Periplasmic solute-binding proteins (SBPs) specific for chitooligosaccharides, (GlcNAc)n (n = 2, 3, 4, 5 and 6), are involved in the uptake of chitinous nutrients and the negative control of chitin signal transduction in Vibrios. Here we propose three-domain mechanism of the (GlcNAc)n translocation based on experiments using a recombinant VcCBP, SBP specific for (GlcNAc)n from Vibrio cholerae. X-ray crystal structures of unliganded or (GlcNAc)3-liganded VcCBP solved at 1.2–1.6 Å revealed three distinct domains, the Upper1, Upper2 and Lower domains for this protein. Based on the crystal structures and molecular dynamics simulation, we here propose that the three domains, Upper1, Upper2, and Lower domains, which correspond to domains I, II, and III, respectively, are required to explain the translocation process of (GlcNAc)2 by CBP.

We solved the structure of unliganded protein (open form) at 1.6 Å, a higher resolution than the VcCBP structures formerly deposited (2.2–2.3 Å resolution). The unliganded form exhibited the largest motion (RMSD, 0.8 nm) of the entire protein molecule, while the motions of the individual domains remained at lower levels (RMSD, 0.1–0.3 nm). This clearly indicated a domain motion, in which the individual domains did not change their own conformations but changed their relative arrangement. In unliganded VcCBP, essential subspaces were widely extended as compared with the liganded VcBP (eigenvector1/eigenvector, -7 ~ 15 nm/-22 ~ 9 nm) revealing a large conformational change from the open state to the closed state. In unliganded VcCBP, strong self-positive correlations (red) were found in the region of residue No. 1-239, which corresponds to Upper1 + Upper2 domains, and also in residue No. 350-440, which includes amino acid residues interacting with the ligand from Lower domain. However, strong inter-negative correlations (blue) were found between 1 and 239 (Upper1 + Upper2) and 350–440 (the interacting region of Lower domain). Furthermore, inter-correlations between 140 and 239 (inner Upper1) and 1–35 (N-terminal Upper1) were rather positive (red). It was clear that Upper1 and Upper2 domains move unitedly in the unliganded state, but that these two domains move independently in the (GlcNAc)3-liganded state.

>[2x]MHHHHHHRSELTIVPDFYPTMVRNFNPYLATNLRTTTDFIYEPLVVFNEMKGNTPVFRLAESYKMADDLMSVTFDIRKGVKWSDGEAFTADDVVYSFGLLKAKPELDQRGINKWVTSVEKVDEYKVRFRLSEANSNVPYEISLIPIVAEHVWKDVKDPTTFTNENPVGTGPFTVIDTFTPQLYIQCRNPNYWDAANLEVDCLRVPQIANNDQLLGKIVNSELDWTSSFVPDIDRTYAAANPNHHYWYPAAGTQAFMVNFKNPDPAKKEALDNVDFRRAFSMALDRQTIIDIAFYGSGTVNDFASGLGYAFEAWSDEATHKKYKGFNTYDVEGSKKLLAKAGFKDVNGDGFVETPSGKSFELLIQSPNGWTDFNNTVQLAVEQLQEVGIKAKARTPEFAVYNQAMLEGTYDVAYTNYFHGADPFTYWNSGYNSALQSGDGMPRFAMHYFTDKKLDGLLDSFYKTADKNEQLAIAHGIQKIIAENQVTIPVMSGAWMYQYNTTRFTGWWSEENPKGRPSVWAGIPERLLHVLDLKPVK> MRPVARLPLSRVLSGCRGFHSQHRTPVLPQVPAAEVQQAASESKVRVAYLLHRQPVVKPTPHPLEMEMAFLLQREHQRYSRHESSESATHFMAQRGQSIDALNRTDPRQIQ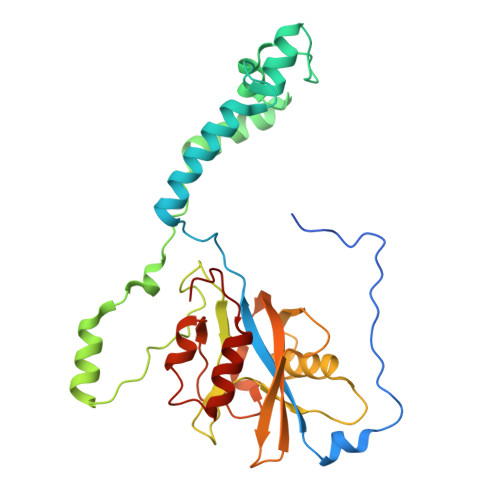SNFFGLELYQDAMRVVLQRYKPERRVTPRDLWDPATYGSSNANSNASSPPTRHSLHRKLDDYLHLIVRDEASGKWTVPQTELRGRETLRMAAERAIATDNGEGLDCYVWSNAPQATVPNANDGSWLFIYVATYLSGRPKFSEFRPKTIDHAWVTRHEMMQYEENFQSPELVRVLLDISADSTFES>[2x]MKFFVQHPYKERIELNIGAITQIV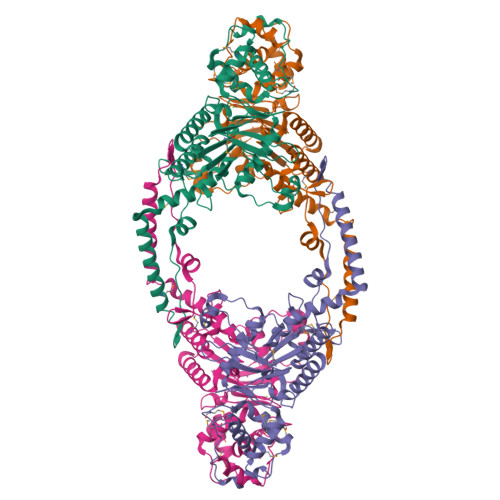GQNNELKYYTWQILSWYFGGKKYSSEDLSIFDYEEPTILDEAREIVKRSSYHYIDISSFKDLLEQMEYKKGTLAQGYLRKIVNQVDIVGHLEKINEQVELIEEAMNRHINLNCGQVEYHLENLPLTLDQLLTKNFSPFFAIENKNLSFEWVSNIDKLSLFLEMLDHLLSQTTEKYLIVLKNIDGFISEESYTIFYRQICHLVKKYPNLTFILFPSDQGYLKIDEENSRFVNILSDQVEHLYDVEFMYERVMKYYPSNDFPTREGFRMSLETVTPYLLTKMLRQPSLSLVDSVILNILNQLFHFSYRIRCSQTPDKELLQKFLESKD>EAPYASLTEIEHLVQSVCKSYRETCQLRLEDLLRQRSNIFSREEVTGYQRKSMWEMWERCAHHLTEAIQYVVEFAKRLSGFMELCQNDQIVLLKAGAMEVVLVRMCRAYNADNRTVFFEGKYGGMELFRALGCSELISSIFDFSHSLSALHFSEDEIALYTALVLINAHRPGLQEKRKVEQLQYNLELAFHHHLCKTHRQSILAKLPPAGKLASLCSQHVERLQIFQHLHPIVVQAAFPPLYKELFSTETESPVGLSK[4x];>TNMGLEAIIRKALMGKYDQWEE[4x]

Retinoic acid-related orphan receptor gamma (RORγ) is a key transcription factor and a master regulator of the differentiation of Th17 cells and the cytokine production. T helper 17 (Th17) cells, which are a subset of CD4+ cells differentiated from naïve T cells, produces proinflammatory cytokines including interleukin 17 (IL-17). Th17 cells and the cytokine production play a pivotal role in autoimmune disease pathology in psoriasis, inflammatory bowel disease, rheumatoid arthritis and multiple sclerosis. Orally available small-molecule inhibitors of RORγ have been created as a substitute medication for injectable biologics, which impose burdens to patients.

We expected that elucidating the complex structure with compound T would be instructive for designing synthetic inhibitors due to a different chemotype from compound A. Therefore, the ternary complex of RORγ-LBD with compound T and CoR peptide was determined at 2.6 Å resolution. As no crystals grew under the previous reservoir conditions for the RORγ-LBD, rockogenin crystals were soaked with compound T and CoR peptide. Extensive interactions of compound T with RORγ-LBD include a direct hydrogen-bonding and van der Waals (VdW) contacts. O atom in the amide group of compound T accepts a hydrogen-bonding from backbone N atom of Glu379. An amide group of compound T orientates towards the opening of the ligand binding pocket with tert-butyl-pyrazole group lying in the hydrophobic residues lining the pocket. Compound T is found to reduce efficacy in the FRET-based CoR recruitment assay. This ternary complex structure reveals the structural mechanism for the decreased CoR recruitment activity of RORγ in the presence of compound T when compared to compound A. The complex structure shows that the binding of compound T induces a movement of helix 5 (H5) that resulted in a decreased interaction interface between CoR peptide and the binding groove of RORγ-LBD. The observed N-terminus region upstream from Glu2351 is unwound and Leu2350 backbone shifts approximately 2 Å outwards from RORγ-LBD. Ile2354 and Leu2358 interact hydrophobically with RORγ-LBD, but Leu2350 does not. Compound T induces the dislocated N-terminus of CoR peptide in a binding mode that will induce less interaction with hRORγ-LBD than that with compound A.>MRPPFTYATLIRWAILEAPEKQRTLNEIYHWFTRMFAFFRNHPATWKNAIRHNLSLHKCFVRVESEKGAVWTVDELEFRKKR[4x];>[2x]SSVPLEWPLSSQSGSYELRIEVQPKPHHRAHYETEGSRGAVKAPTGGHPVVQLHGYMENKPLGLQIFIGTADERILKPHAFYQVHRITGKTVTTTSYEKIVGNTKVLEIPLEPKNNMRATIDCAGILKLRNADIELRKGETDIGRKNTRVRLVFRVHIPESSGRIVSLQTASNPIECSQRSAHELPMVERQDTDSCLVYGGQQMILTGQNFTSESKVVFTEKTTDGQQIWEMEATVAAAAAAPNMLFVEIPEYRNKHIRTPVKVNFYVINGKRKRSQPQHFTYHP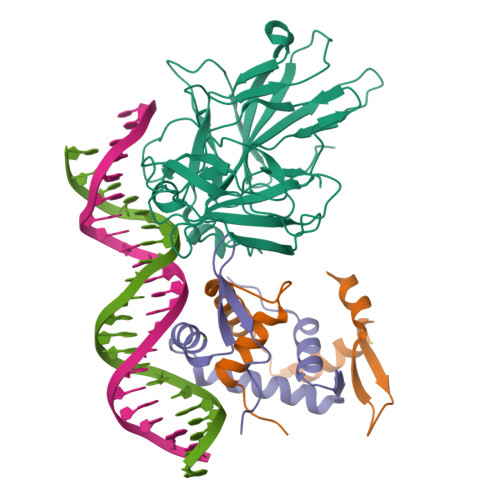V>[2x]MRRYEVNIVLNP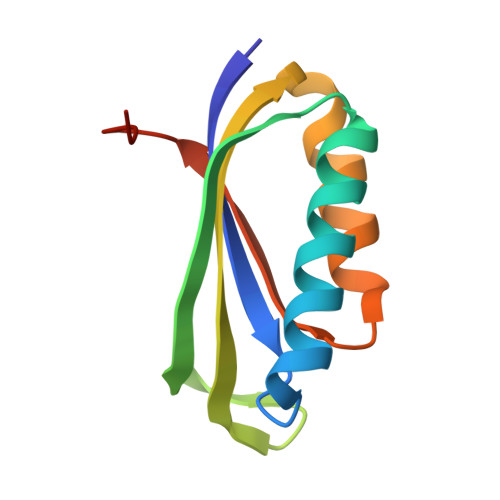NLDQSQLALEKEIIQRALENYGARVEKVAILGLRRLAYPIAKDPQGYFLWYQVEMPEDRVNDLARELRIRDNVRRVMVVKSQEPFLANA>[2x]GSHMNINKQSPIPIYYQIMEQLKTQIKNGELQPDMPLPSER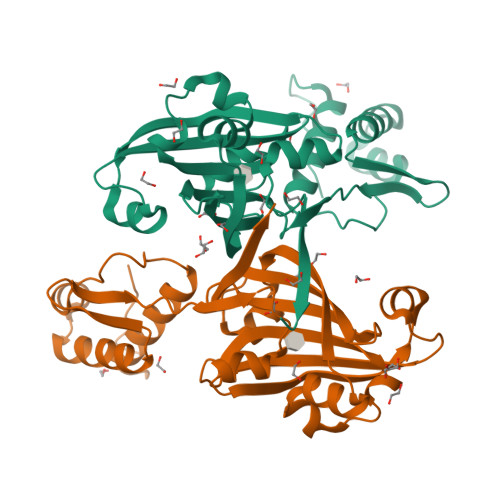EYAEQFGISRMTVRQALSNLVNEGLLYRLKGRGTFVSKPKMEQALQGLTSFTEDMKSRGMTPGSRLIDYQLIDSTEELAAILGCGHPSSIHKITRVRLANDIPMAIESSHIPFELAGELNESHFQSSIYDHIERYNSIPISRAKQELEPSAATTEEANILGIQKGAPVLLIKRTTYLQNGTAFEHAKSVYRGDRYTFVHYMDRLS> AARYDDILYFPAS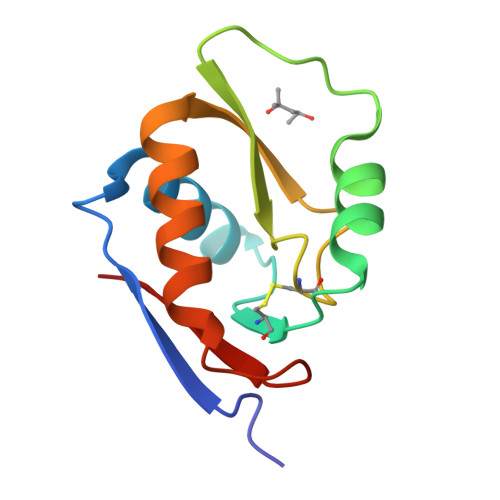RYPETGAHISDAIKAGHSDVCTIERSGADKRRQESLKGIPTKPGFDRDEWPMAMCEEGGKGASVRYVSSSDQRGAGSWVGNRLSGFADGTRILFIVQ The LarA family consists of diverse racemases/epimerases that interconvert the diastereomers of a variety of α-hydroxyacids by using a nickel-pincer nucleotide (NPN) cofactor. Accumulating evidence has supported a proton-coupled hydride transfer (PCHT) mechanism for the LarA-catalyzed racemization reaction. According to this hidden redox reaction mechanism, the hydrogen atom on Cα of lactate is transferred as a hydride to the NPN cofactor and then, after a rotation of the acetyl group of the pyruvate intermediate, the hydride returns to Cα to complete racemization. In this work, we report the high-resolution crystal structures of LarA from Isosphaera pallida (LarAIp) in complex with three short-chain aliphatic D-α-hydroxyacids.

To address this problem, we applied a heating-cooling treatment to promote ligand exchange. In the heating step, the purified protein was incubated with a non-D-lactate substrate at approximately 3 mM at 55 °C for 15 min. In this step, the increased dynamics of the protein at the elevated temperature leads to the opening of the active site to the solvent, allowing the release of the bound D-lactate and the binding of the alternative substrate to the active site. In the cooling step, the temperature was changed rapidly to 4 °C in a thermal cycler, followed by incubation on ice to lock the conformation in the most stable state. It should be noted that D/L-2HB was used in the ligand exchange experiment but only the D-enantiomer was found to be bound in the active site. The two D-substrates adopt the same orientation as D-lactate and interact with the same set of residues in the active site. Importantly, the aliphatic substituents on Cα of all three substrates point to the same space that is defined by Leu174, Met175, Trp356, and Gln357. In both structures, the amide group in the side chain of Gln357 in Conformation A moves away from the substrate by approximately 0.4 Å, and Conformation B leaves more space to accommodate the substrates with a larger Cα substituent. This result indicates that Gln357 exclusively confers the plasticity of the active site. The geometry and the hydrophobic nature of the substrate binding pocket defined by these residues, as well as the flexibility of Gln357, explained the negative correlation between the size and polarity of the Cα substituents and the reactivity of the substrates.

> ARVTLDYGKTGLNVDLPDDRTLPPLTIRPAPPLDDPEAEVVRCLAEPIGSPPLLDLARGKRSACILVCDITRPVPNPVLLRPILRTLHAAGLATQDILILVATGLHRPSTPAEKVEMLSEEIARTYRVEDHYGTRLEEHTYLGTTPNGVPAWIDSRYVQADLKIATGLIEPHLMAGYSGGRKLICPGIAAFETVKLWHGPRFLEHPLADCGFLEGNPVHEENTRIARMAGCDFIVNVTLDGARRITSVVAGDMEQAFLKGVAFVETVVKAAVPAPVDVVVTSSAGHPLDLTFYQAVKGLTGALPIVKPGGTIVIAAALAEGLGSPEFQSLFEEHPTLEGFMEAILKEESFTVDQWQLEELAKVRRKARVKFVSDGVPAAVLSRCHVEPVATVELAVAQALEQYGPEARVAVIPKGPYVLPVVDPT5-BROMO-URIDINE-5'-MONOPHOSPHATE | C9 H12 Br N2 O9 P | 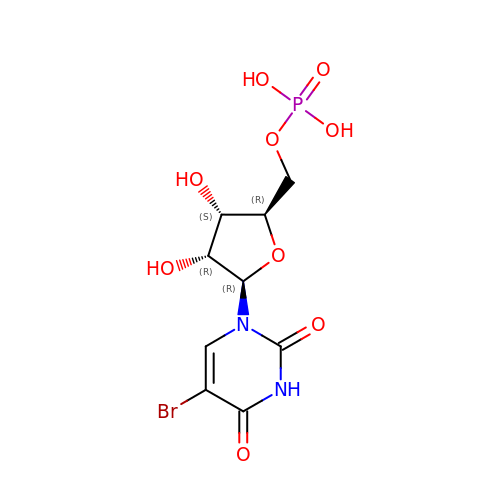IDPVUMJNEZFMNU-UAKXSSHOSA-N> MSALLSQASGFSGLALGSSASSKRLCKPLCRRPAVCVQAAHRPASAVSSGVPSTGFGPVSPLQRRPTLPTRKLVVASSQSGGRAEDAEKQDWKFGRNEGPMTWPWKLMCAILYMLPWVDVTEKTVYFVERFPAFVWTEYFSEPFEHWYNIHEYAPLFIFFATYLGIVRNKKIPHVARYHVMMGVMLDIVAMILIVTEENLPTGVLW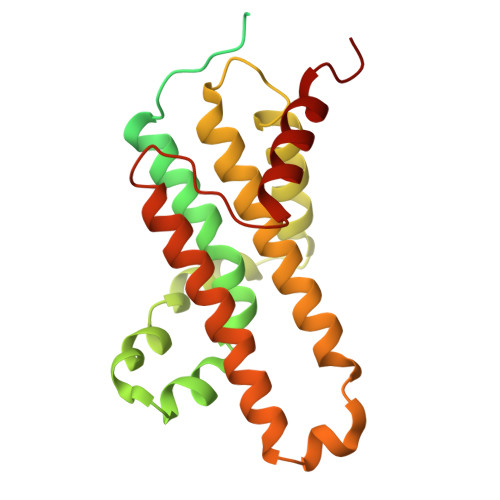TPWSDLFYALMFWFIFLLVIYCLFFCFLGWYCEIPLISEGVYLQIEQAEQLGQ> WELTILHTNDVHSRLEQTSEDSSKCVDASRCMGGVARLFTKVQQIRRAEPNVLLLDAGDQYQGTIWFTVYKGAEVAHFMNALRYDAMALGNHEFDNGVEGLIEPLLKEAKFPILSANIKAKGPLASQISGLYLPYKVLPVGDEVVGIVGYTSKETPFLSNPGTNLVFEDEITALQPEVDKLKTLNVNKIIALGHSGFEMDKLIAQK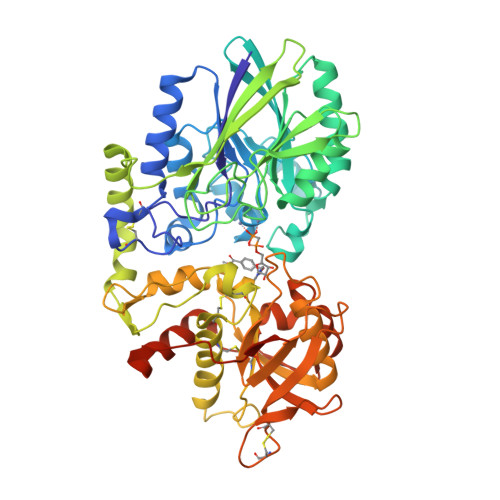VRGVDVVVGGHSNTFLYTGNPPSKEVPAGKYPFIVTSDDGRKVPVVQAYAFGKYLGYLKIEFDERGNVISSHGNPILLDSSIPEDPSIKADINKWRIKLDDYSTQELGKTIVYLDGSSQSCRFRECNMGNLICDAMINNNLRHTDEMFWNHVSMCILNGGGIRSPIDERNDGTITWENLAAVLPFGGTFDLVQLKGSTLKKAFEHSVHRYGQSTGEFLQVGGIHVVYDLSRKPGDRVVKLDVLCTKCRVPSYDPLKMDEVYKVILPNFLANGGDGFQMIKDELLRHDSGDQDINVVSTYISKMKVIYPAVEGRIKFSGGGGAGGGGGTKHHHHHH>[2x]MIDLLQADGNALPSAVKLAYSPASKTFESYRVMTQVHTNDATKKVIVKLADTPQLTDVLNSTVQMPISVSWGGQVLSTTAKEFEAAALGYSASGVNGVSSSQELVISAAPKTAGTAPTAGNYSGVVSLVMTLGSDNKQVEKNITVTASVDPVIELLQADGNALPSAVKLAY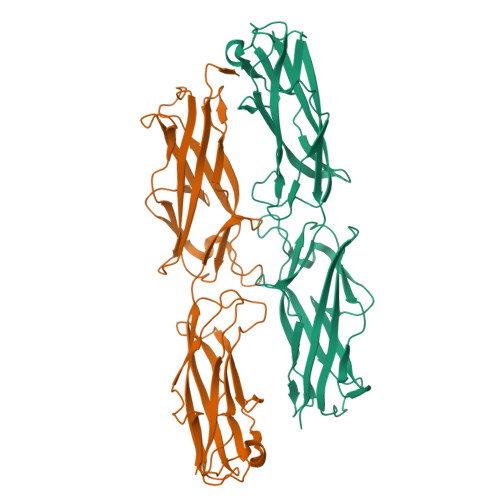SPASKTFESYRVMTQVHTNDATKKVIVKLADTPQLTDVLNSTVQMPISVSWGGQVLSTTAKEFEAAALGYSASGVNGVSSSQELVISAAPKTAGTAPTAGNYSGVVSLVMTLGSDNKQVEKNITVTASVDPVILEHHHHHH>MKHHHHHHPMVKEYKTITQIAGPLIFVEKTEPVGYNEIVNIKMGDGTVRRGQVLDSSADIVVVQVFEGTGGLDKDCGVIFTGETLKLPASVDLLGRILSGSGEPRDGGPRIVPDQLLDINGAAMNPYARLPPKDFIQTGISTIDGTNTLVRGQKLPIFSASGLPHNEIALQIARQASVPGSESAFAVVFAAMGITNEEAQYFMSDFEKTGALERAVVFLNLADDPAVERIVTPRMALTAAEYLAYEHGMHVLVILTDITNYAEALRQMGAARNEVPGRRGYPGYMYTDLATLYERAGIVKGAKGSVTQIPILSMPGDDITHPIPDLSGYITEGQIVVARELHRKGIYPP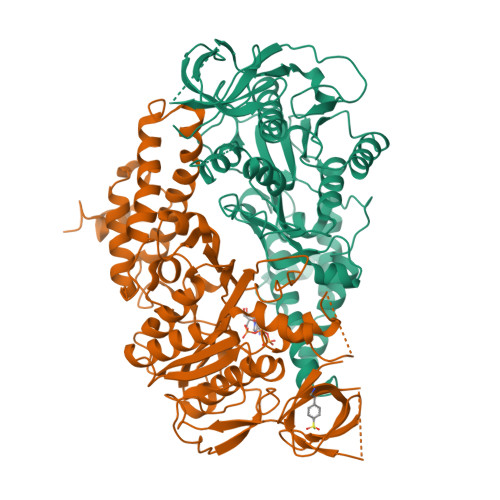INVLPSLSRLMNSGIGAGKTREDHKAVSDQMYAGYAEGRDLRGLVAIVGKEALSERDTKFLEFADLFEDKFVRQGWNENRTIEDTLEIGWQILTHLPENQLGRIDNKYIQKYHPAHRKAK[2x]>[2x]GAHMSGRMTDDKDVLRDVWFGRIPTCFTLYQDEITEREAEPYYLLLPRVSYLTLVTDKVKKHFQKVMRQEDISEIWFEYEGTPLKWHYPIGLLFDLLASSSALPWNITVHFKSFPEKDLLHCPSKDAIEAHFMSCMKEADALKHKSQVINEMQKKDHKQLWMGLQNDRFDQFWAINRKLMEYPAEENGFRYIPFRIYQTTTERPFIQKLFRPVAADGQLHTLGDLLKEVCPSAIDPEDGEKKNQVMIHGIEPMLETPLQWLSEHLSYPDNFLHISIIPQPTD;>[2x]GGGRPRWKRHISEQLRRRDRLQRQAFEEIILQYNKLLEKSDLHSVLAQKLQAEKHDVPNRHEISPGHDGTWNDNQLQEMAQLRIKHQEELTELHKKRGELAQLVIDLNNQMQRK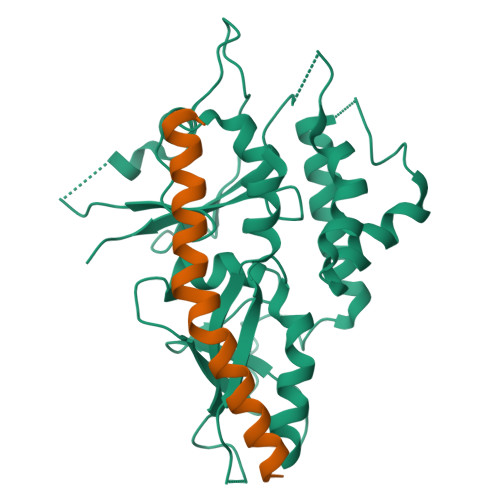DREMQMNEAKIAECLQTISDLETECLDLRTKLCDLERANQTLKDEYDALQITFTALEGKLRKTTEENQELVTRWMAEKAQEANRLNAENEKDSRRRQARLQKELAEAAKEPLPVEQDDDIEVIVDETSDHTEETSPVRAISRAATKRLSQPAGGLLDSITNIFGRRSVSSFPVPQDNVDTHPGSGKE>[3x]NYLDLFSHKNMKLKERVLIPVKQYPKFNFVGKILGPQGNTIKRLQEETGA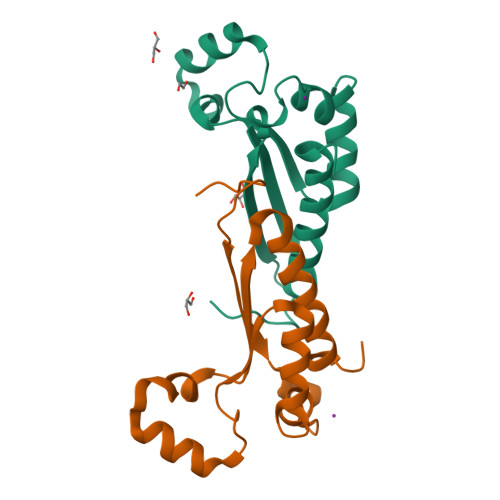KISVLGKGSMRDKAKEEELRKGGDPKYAHLNMDLHVFIEVFGPPCEAYALMAHAMEEVKKFLVPDM> GPGSKPFTLPILTIGELTNSRFPVPIDELYTSPNESLVVQPQNGRCALDGELQGTTQLLPTAI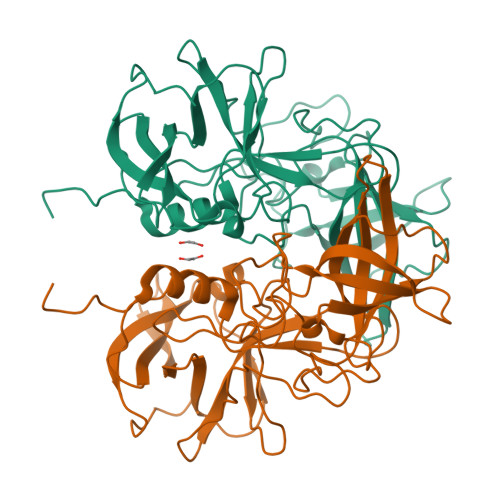CSFRGRINQKVSGENHVWNMQVTNINGTPFDPTEDVPAPLGTPDFSGKLFGVLSQRDHDNACRSHDAVIATNSAKFTPKLGAIQIGTWEEDDVHINQPTKFTPVGLFEDGGFNQWTLPNYSGALTLNMGLAPPVAPTFPGEQILFFRSHIPLKGGVADPVIDCLLPQEWIQHLYQESAPSQSDVALIRFTNPDTGRVLFEAKLHRSGYITVANTGSRPIVVPANGYFRFDSWVNQFYSLAPM> GPKLSLIKVVNGCRLGKIQNLGKAGDCTVDIPGCLLYTRTGSAPHLTHQTLRNIHGVPGIAQLTLSSLAEHHEVLAEYKKGVGSFIGMPESLFYCSLHDPVTPGPAGYVTSKSVSVWGFGGRVEMTVSKFMAIQEALQPDWFQCLSDGEASCAETTSIKRARKSVDRSLLFLDSCLRLQEESEVLQKSVIIGVIEGGDVMEERLRSARETAKRPVGGFLLDGFQGDPAVTETRLHLLSSVTAELPEDKPRLICGVSRPDEVLECIERGVDLFESF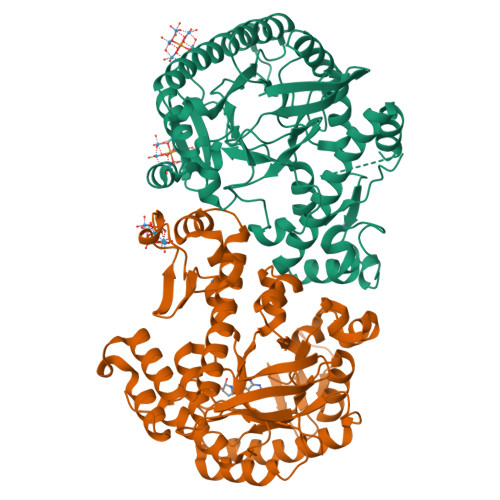FPYQVTERGCALTFTFDCQLNPEETLLQQNGIQEKIKGLDQAKKIEATGCNQEMTSFEINLKEKKYQEDFDPLVRGCSCYCCKNHTRAYIHHLLMTNELLAGVLLMMHNFEHYFGFFCSIREALKNDTLAQLKELICRQMFDNN;> GPESAPRIMRLVAECSRSGARAGELRLPHGTVATPVFMPVGTQATMKGITTEQLDSLGCRICLGNTYHLGLRPGPELIRKAQGLHGFMNWPHNLLTDSGGFQMVSLFSLSEVTEEGVHFRSPYDGEETLLSPERSVEIQNALGSDIIMQLDHVVSSTVTGPLVEEAMHRSVRWLDRCIAAHKHPDKQNLFAIIQGGLNADLRTTCLKEMTKRDVPGFAIGGLSGGESKAQFWKMVALSTSMLPKDKPRYLMGVGYATDLVVCVALGCDMFDCVYPTRTARFGSALVPTGNLQLKKKQYAKDFSPINPECPCPTCQTHSRAFLHALLHSDNTTALHHLTVHNIAYQLQLLSAVRSSILEQRFPDFVRNFMRTMYGDHSLCPAWAVEALASVGIMLT>MGPVWRKHYITYRINNYTPDMNREDVDYAIRKA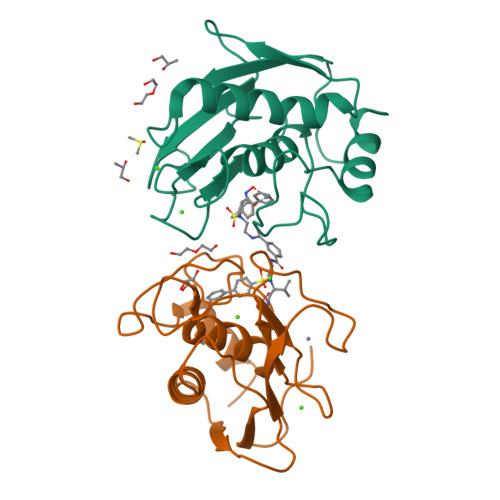FQVWSNVTPLKFSKINTGMADILVVFARGAHGDDHAFDGKGGILAHAFGPGSGIGGDAHFDEDEFWTTHSGGTNLFLTAVHEIGHSLGLGHSSDPKAVMFPTYKYVDINTFRLSADDIRGIQSLYG[4x]1-(2-methylsulfanylphenyl)piperazine | C11 H16 N2 S | 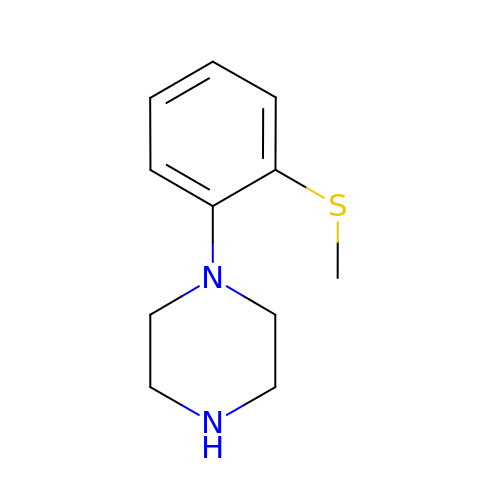RXJURXTXLCOIDY-UHFFFAOYSA-N> MHFETVIGLEVHVELKTDSKMFSPSPAHFGAEPNSNTNVIDLAYPGVLPVVNKR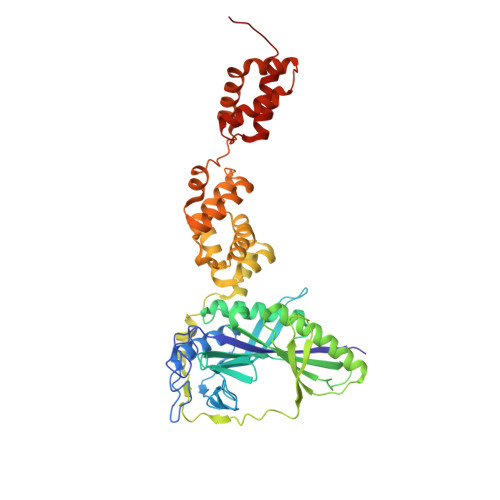AVDWAMRAAMALNMEIATESKFDRKNYFYPDNPKAYQISQFDQPIGENGYIDIEVDGETKRIGITRLHMEEDAGKSTHKGEYSLVDLNRQGTPLIEIVSEPDIRSPKEAYAYLEKLRSIIQYTGVSDVKMEEGSLRCDANISLRPYGQEKFGTKAELKNLNSFNYVRKGLEYEEKRQEEELLNGGEIGQETRRFDESTGKTILMRVKEGSDDYRYFPEPDIVPLYIDDAWKERVRQTIPELPDERKAKYVNELGLPAYDAHVLTLTKEMSDFFESTIEHGADVKLTSNWLMGGVNEYLNKNQVELLDTKLTPENLAGMIKLIEDGTMSSKIAKKVFPELAAKGGNAKQIMEDNGLVQISDEATLLKFVNEALDNNEQSVEDYKNGKGKAMGFLVGQIMKASKGQANPQLVNQLLKQELDKRLEHHHHHH> GSGMEQFPKETVVESSGPKVLETAEEIQERRQEVLTRYQSFKERVAERGQKLEDSYHLQVFKRDADDLGKWIMEKVNILTDKSYEDPTNIQGKYQKHQSLEAEVQTKSRLMSELEKTREERFTMGHSAHEETKAHIEELRHLWDLLLELTLEKGDQLLRAL;> GSTADKFRFFSMARDLLSWMESIIRQIETQERPRDVSSVELLMKYHQGINAEIETRSKNFSACLELGESLLQRQHQASEEIREKLQQVMSRRKEMNEKWE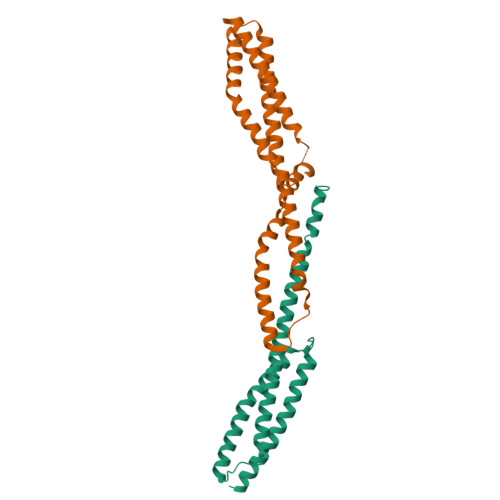ARWERLRMLLEVCQFSRDASVAEAWLIAQEPYLASGDFGHTVDSVEKLIKRHEAFEKSTASWAERFAALEKPTTLELKERQIAER>[4x]MAEKPKLHYFNARGRMESTRWLLAAAGVEFEEKFIKSAEDLDKLRNDGYLMFQQVPMVEIDGMKLVQTRAILNYIASKYNLYG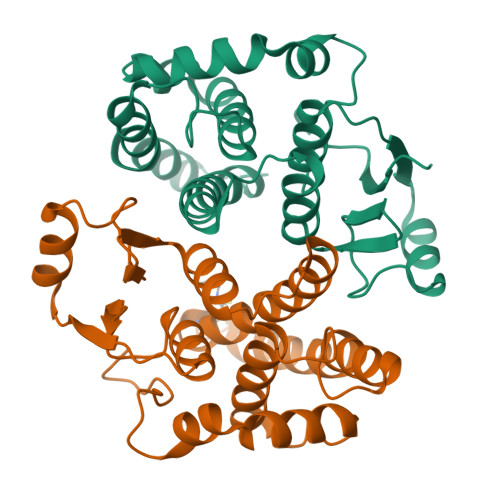KDIKERALIDMYIEGIADLGEMILLLPVCPPEEKDAKLALIKEKIKNRYFPAFEKVLKSHGQDYLVGNKLSRADIHLVELLYYVEELDSSLISSFPLLKALKTRISNLPTVKKFLQPGSPRKPPMDEKSLEEARKIFRF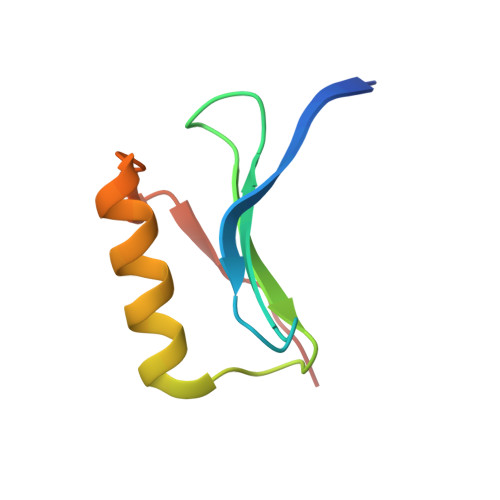> MGPFYGGYNVIALDREYRHALVCGPDRDYLWILSRTPTISDEVKQEMLAVATREGFDVSKFIWVQQPGS[(2~{R})-pyrrolidin-2-yl]methyl ~{N}-[(3~{S})-2,6-bis(oxidanylidene)piperidin-3-yl]carbamate | C11 H17 N3 O4 | 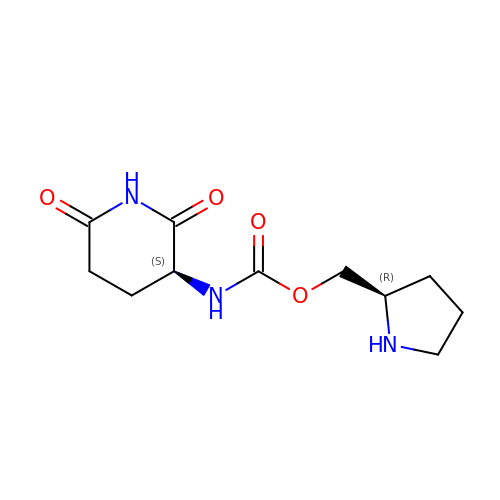UKQUVPXPHSBKIC-SFYZADRCSA-N>MHHHHHHGSKIKKIEPYVISHKLDTPFYFSQWQYDTRKICIVKITLDDGTYGWGEGYGPAAVIKSGIDFFTPFLLGKEAIGHEVLWQEMYRRSMDYARSGVLQAAISAIDVALWDIKGKLLNLPVSVLLGGVKNPIIEPYATGLYFTRTENLEELLVEEALLYKSQGFKATKMKVGLGIEQDLKYIAAI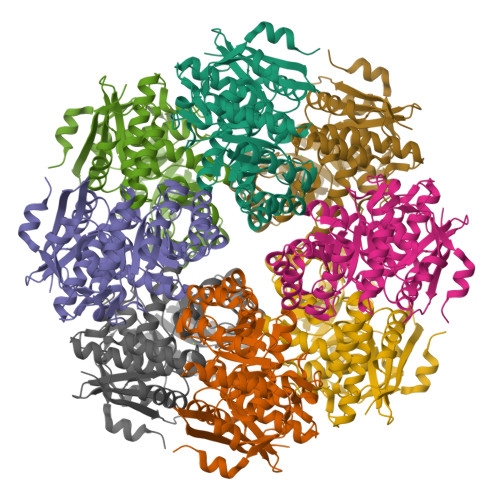RKAIGPDMRLMIDSNHAYCYKEAIELARKAEKFDISWFEEPVSPEDYDGYKRLRQNTTIPISGGECEYLKYGFKRLFDKDCVDIAQPDICAAGGLTEVKKIATLAQTYNVDLVPHTWGTWIAISAAVHLVANLDKNPGRMYNDLPTMELDRTENALRDEVTLHKIKLENGHLEVPCTPGLGVDVDMDKLEHYLDKEIHKDGATKIRS[8x]> ECDFSPLLSGTPPQVYNFKRLVFTNCNYNLTKLLSLFSVND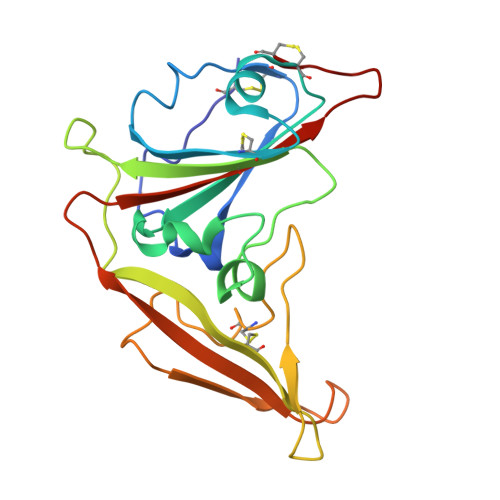FTCSQISPAAIASNCYSSLILDYFSYPLSMKSDLSVSSAGPISQFNYKQSFSNPTCLILATVPHNLTTITKPLKYSYINKCSRLLSDDRTEVPQLVNANQYSPCVSIVPSTVWEDGDYYRKQLSPLEGGGWLVASGSTVAMTEQLQMGFGITVQYGTDTNSVC> GAMGSSPNYDKWEMERTDITMKHKLGGGQYGEVYEGVWKKYSLTVAVKTLKEDTMEVEEFLKEAAVMKEIKHPNLVQLLGVCTREPPFYIITEFMTYGNLLDYLRECNRQEVNAVVLLYMATQISSAMEYLEKKNFIHRDLAARNCLVGENHLVKVADFGLSRLMTGDTYTAHAGAKFPI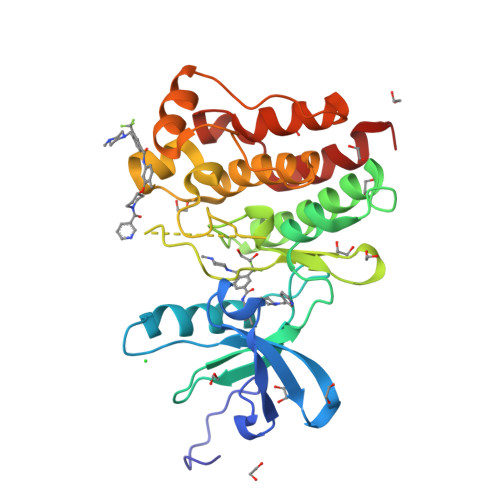KWTAPESLAYNKFSIKSDVWAFGVLLWEIATYGMSPYPGIDLSQVYELLEKDYRMERPEGCPEKVYELMRACWQWNPSDRPSFAEIHQAFETMFQES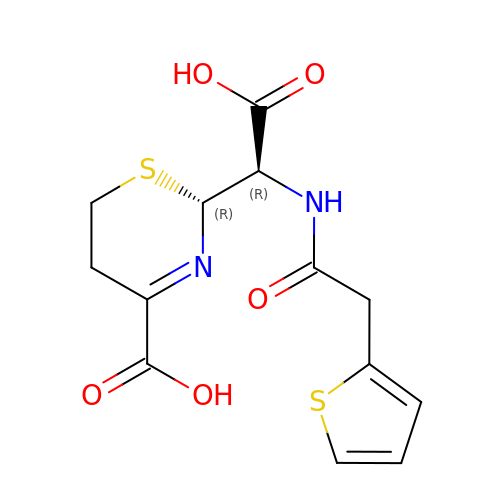(2R)-2-{(1R)-2-OXO-1-[(2-THIENYLACETYL)AMINO]ETHYL}-5,6-DIHYDRO-2H-1,3-THIAZINE-4-CARBOXYLIC ACID | C13 H14 N2 O5 S2 | LNPNJPUNJYVKHH-WDEREUQCSA-N>KAVYLWTVSDVLKWYRRHCGEYTQYEQLFAQH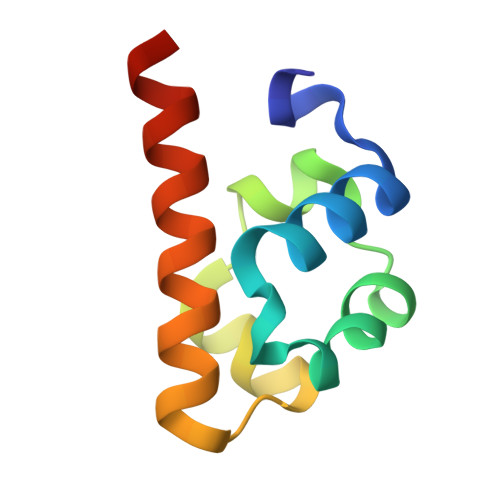DITGRALLRITDSSLQRMGVTDNRDREAIWREIVKQRLKTDIMEIR[2x]>MNSLLRLPALKRGVFTMSKRGLATTVSPKTRTSNLKNGLTIASESNPLVQTATVGVWIDAGSRNENAYNNGTAHFFEHLAFKGTDKRSQHQLELDIENMGGHLNAYTSRESTVYYAKSFKDDVPKSVEILADILQHSKLAESAIDREREVITRELEEVNKQYEEVVFDHLHATAFMNQPLGRTILGPRENIQTITNTELRKFITENYTADRMVLVGAGAVDHDALVELAEKYFSHLPSSQSPVPLGTPRSSGEDANQNPIPNFVGSEVRLRDDTMPVAHIAIAVEGVSWTSEDYYTALVAQAIIGNYDRAVGTSRHQGSRLSNIVSENNLANSFQSFSTSYSDTGLWGIYLTSENTTQIDDLVHFTLKEWNRLSTSVSNLQVERAKSQLKAGLLLSLDGTTYVAEDIGRQLTTLGRRVTPAEVEAKLEAVTEHDVRAWAQKTLYDKDIALVGLGPIEGLYDYNRIRNDMSMMRW[2x];>[2x]MTRGVPRLAVAARHFSTAEAAGVKVAAQDGQSPISDLSVVLRGGSRYATVPGVSHILEKFAFQNTVPKSALRFVRELELFGGKLYTHTTREHIVLRTQFLKQDLPYFVDAFANVLKETKFQQFELTERVAPVAELDLLKRESDPAFTALEAAHEVAFRTGLGNSVYAQGYSPVTLEDVKEFARQVYAKQNVAVVGNNVVPADLQQLVGTAFADLQEGSKVTQAGTTTLHGGEARVRTSTGNALTIALPIAEPKPVYHALASFLGGPASMPWSVGASPLAQATVGTHTSVKATYHNYGDAGLFAITIKGDSPAEISQVAHKAVQALKDTGAEVTEEQAARAYAKSKFAAAEAFENPDSSASVIGMELLSGVSRIAPENVQKFTPAELSEAAAQLSASAKPVVAAVGQVHALPFADELF;>MALRKKNSLLNMANSYVLDSPQPSNLNYFWNFGSLLALCLVIQLATGITLAMHYTSHASLAFDSVEHIMRDVNFGWFIRYAHANTASFFFICIYAHMGRNIYYGSYKTPRVLPWSIGVIIFLLLIITAFMGYVLVFGQMSLWGATVICNLVSAIPWLGEDIVHFLWGGFSVGNPTLQRFFALHYLMPFVLAVFALLHLIALHTAGSSNPLGITSNVDKLSMHPYYSFKDLITVFAFLLMFTLFVFFSPDKLGHPDNYIPANPMVTPASIVPEWYLLPFYAILRAIPDKLGGVIAMVAAILILLILPIVDRSIIRGNAFKPISKLLFGFFICNFLLLGVLGQVHIEPPFIVLGQICTIFYFSYFLILLPMVSTIENIFFYIGSLRK[2x];>MRRRRIGVWPENRRVSRLWVSLSPRSCVTCPVPTNQNPPINNHHTPILTQMFKAIPLRQALLGISSAVCAGATTTYYYTTKAEAMTAAEHGLHPAEYPWPQNGMLSTFDHASLRRGYQVYKEVCAACHSLDRIAWRNLVGVTHTTDEAKAFAEELEYDDEPDDEGNPRKRPGKLADYIPGPYPNEQAARAANQ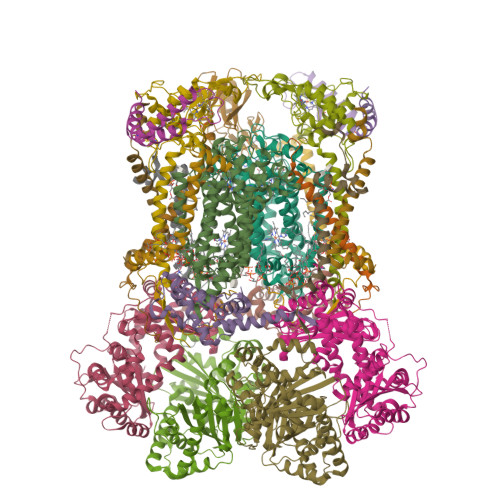GALPPDLSLIAKARHGGADYIFALLTGYPDEPPAGVVLAPGMNYNPYFPGGGIGMARTLFDGVVEYEDGTPATTSQMAKDVAAFLTWAAEPEHDERKKLGLKAIIVISAMLGLSVYIKKFKWSPIKNRKFIYNPPKN[2x];>MSLLRTAAQAVKAPKAYTPLVAAKAFAQTRSVSSQPIGGKSTYKIPDFTPYLKKDRNTDANRLFSYFMIGSFGMLSAAGAKATVQDFLSNMSASADVLAMAKVEVKLGAIPLGKNVIIKWRGKPIFIRHRTSEEIEEANEVNVATLRDPQTDDERVQKPEWLVMIGVCTHLGCVPIGEAGDFGGWFCPCHGSHYDISGRIRRGPAPLNLEIPEYDFADAETLVIG[2x];>[2x]MSYFLTLASEVAESLLPTVAFASEEEKEQDEPVEVESDDDESEEKEDDDEEEDEDDDDDDDDDEVPDPAIALHEAAAEGPCHDFKHHFDECVERVTKAQEAEDYDHAEYKEDCVEEFFHLQHCINDNTADKLFRVLK;>[2x]MASITSVVKTSELILKSPLLSKIVVPLAKTYVKFSGYRQLGFKMNDLIIEETPNMQLALRRLPPTESYDRVYRLIRATQFSLSHKLATGNDITKPEEDDHYLIPYILDVEAEAFEKDALDNLEVVKRK;>MGGNGHYMGWWGHMGSPPQKGIAGYTISPFAARPFAGVVHAAIFNTFRRTKNQALFVILPVSFFYYVWTQASEKNEWLYTKAGRHELAKALAE[2x];>MAWATTFYNVFVKRNSAFVATILASAFVFDMTFETAIDNFWDRINAGKQWKDIRHKYIEAAGDDDEDDE[2x];>MICGEGDYVKKPSYKIVPHFLGFNIPTVSKWIPIFGIWGAAAGIGALFLIEGVPRTRQDILSKIPIIGEHWIREIPASDNPF[2x]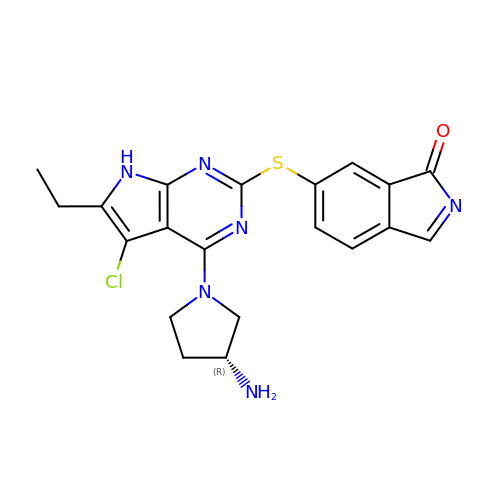6-({4-[(3R)-3-aminopyrrolidin-1-yl]-5-chloro-6-ethyl-7H-pyrrolo[2,3-d]pyrimidin-2-yl}sulfanyl)-1H-isoindol-1-one | C20 H19 Cl N6 O S | MFHNBYVWNDLIQC-LLVKDONJSA-N>[2x]MHRTSNGSHATGGNLPDVASHYPVAYEQTLDGTVGFVIDEMTPERATASVEVTDTLRQRWGLVHGGAYCALAEMLATEATVAVVHEKGMMAV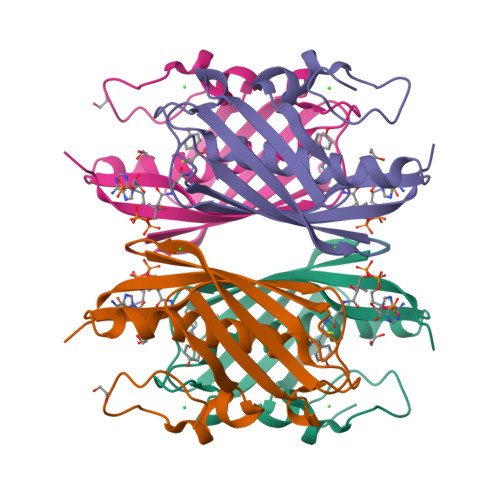GQSNHTSFFRPVKEGHVRAEAVRIHAGSTTWFWDVSLRDDAGRLCAVSSMSIAVRPRRD> MTTATIEE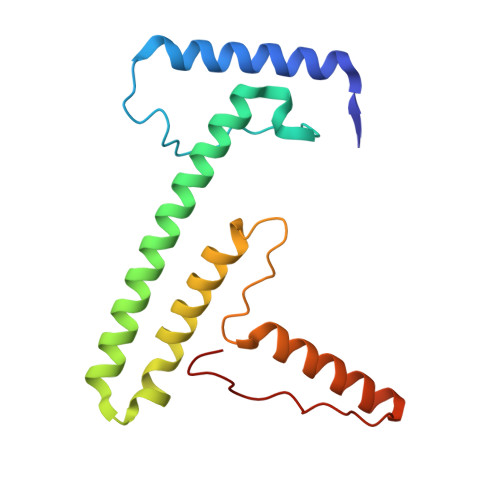RRAFHKEVLDIVQSKLANKNSEWARPEEPILHNLKSEKEEPHVYYHNNNFRVTRQLIHFEKTKIFEDELDKCMRTHGEAKYRKCQEIAKRFQASCRVASNLERGPNARKRDVGFIYQNNKLRELEKDAKELGLNNPFPPSSPRTTIGY1-biotinylpyrene 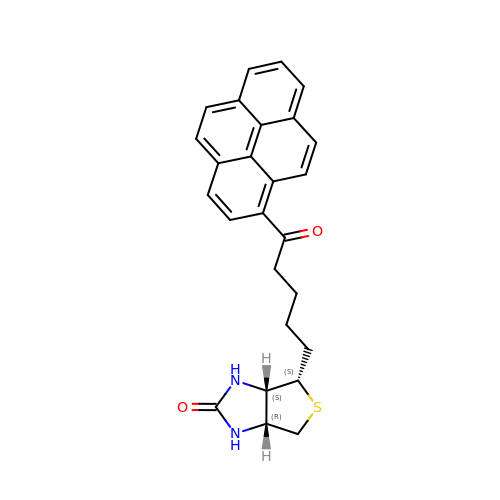| C26 H24 N2 O2 S | AKVNOAJJWXUFFK-XTJBDQBJSA-N> MASMTGGQQMGRDEAGITGTWYNQLGSTFIVTAGADGALTGTYESAVGAAESRYVLTGRYDSAPATDGSGTALGWTVAWKNNYRNAHSATTWSGQYVGGAEARINTQWLLTSGTTEANAWKSTLVGHDTFTKVKPSAASID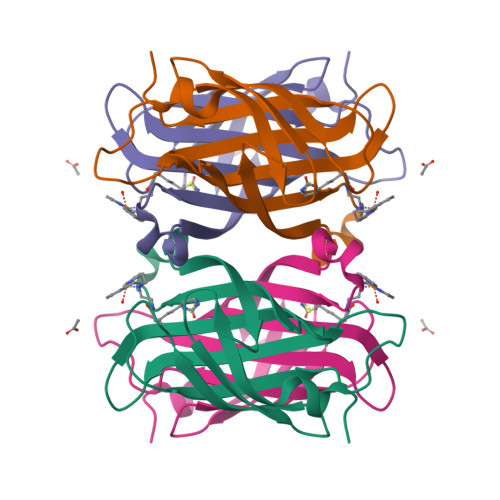AAKKAGVNNGNPLDAVQQ beta-D-allofuranose | C6 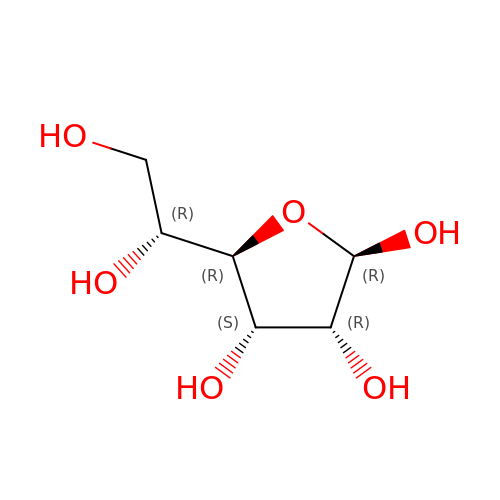H12 O6 | AVVWPBAENSWJCB-AIECOIEWSA-N>MTIFDNYEVWFVIGSQHLYGPETLRQVTQHAEHVVNALNTEAKLPCKLVLKPLGTTPDEITAICRDANYDDPCAGLVVWLHTFSPAKMWINGLTMLNKPLLQFHTQFNAALPWDSIDMDFMNLNQTAHGGREFGFIGARMRQQHAVVTGHWQDKQAHERIGSWMRQAVSKQDTRHLKVCRFGDNMREVAVTDGDKVAAQIKFGFSVNTWAVGDLVQVVNSISDGDVNALVDEYESCYTMTPATQIHGEKRQNVLEAARIELGMKRFLEQGG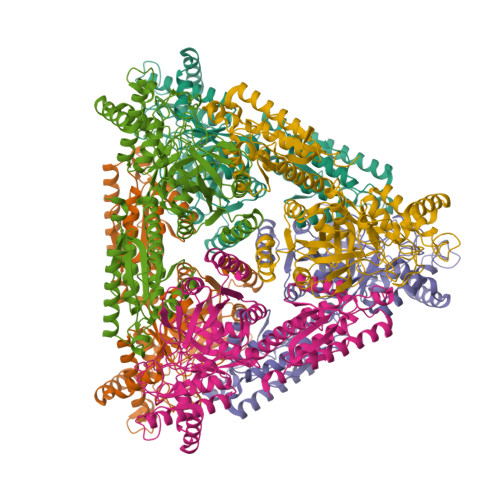FHAFTTTFEDLHGLKQLPGLAVQRLMQQGYGFAGEGDWKTAALLRIMKVMSTGLQGGTSFMEDYTYHFEKGNDLVLGSHMLEVCPSIAVEEKPILDVQHLGIGGKDDPARLIFNTQTGPAIVASLIDLGDRYRLLVNCIDTVKTPHSLPKLPVANALWKAQPDLPTASEAWILAGGAHHTVFSHALNLNDMRQFAEMHDIEITVIDNDTRLPAFKDALRWNEVYYGFRR[3x]> MSENSEIMKYVATTCPYCGVGCTLNLVVSNGKVVGVEPNQRSPINEGKLCPKGVTCWEHIHSPDRLTTPLIKKDGKFIEASWDEALDLVAKNLKVIYDKHGPKGLGFQTSCRTVNEDCYIFQKFARVGFKTNNVDNCARICHGPSVAGLSLSFGSGAATNGFEDALNADLILIWGSNAVEAHPLAGRRIAQAKKKGIQIIAVDPRYTMTARLADTYVRFNPSTHIALANSMMYWIIKEGLEDKKFIQDRVNGFEDLKKTVENYADAEAIHGVPLDVVKDIAFRYAKAKNAVIIYCLGITELTTGTDNVRSMGNLALLTGNVGREGVGVNPLRGQNNVQGACDMGAYPNVYSGYQKCEVAENRAKMEKAWSVTNLPDWYGATLTEQINQCGDEIKGMYILGLNPVVTYPSSNHVKAQLEKLDFLVVQDIFFTETCQYADVILPGACFAEKDGTFTSGERRINRVRKAVNPPGQAKEDIHIISELAAKMGFKGFELPTAKDVWDDMRAVTPSMFGATYEKLERPEGICWPCPTEEHPGTPILHREKFATA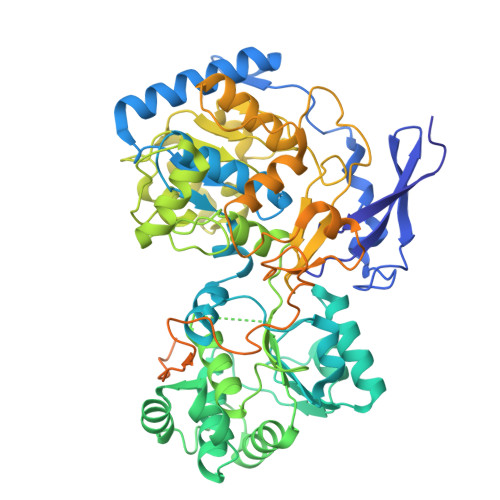DGKGNLFGIDYRPPAEVADAEYPFTLMTGRLIFHYHSRTQTDRAADLHREVPESYAQINIEDARRLGIKNNEYIKLKSRRGETTTLARVTDEVAPGVVYMTMHFADGVNNLTNTVLDPMSKMPELKHCAISIEKVGGN> MAMQAAKRANIR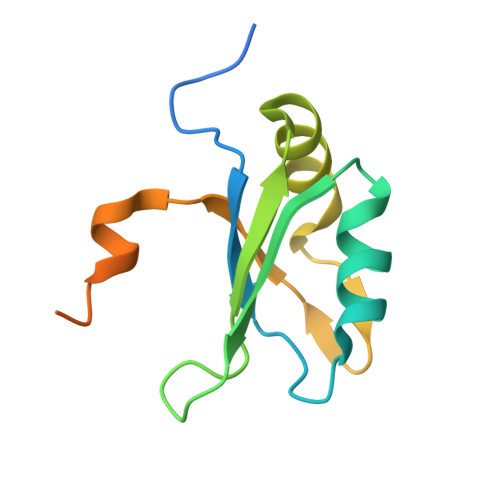LPPEVNRILYIRNLPYKITAEEMYDIFGKYGPIRQIRVGNTPETRGTAYVVYEDIFDAKNACDHLSGFNVCNRYLVVLYYNANRAFQKMDTKKKEEQLKLLKEKYGINTDPPK> MGSSKPLKGFVICCTSIDLKQRTEISTKATKLGAAYRSDFTKDVTHLIAGDFDTPKYKFAAKSRPDIKIMSSEWIPVLYESWVQGEDLDDGLLVDKHLLPTLFKCRVCLTNIGQPERSRIENYVLKHGGTFCPDLTRDVTHLIAGTSSGRKYEYAL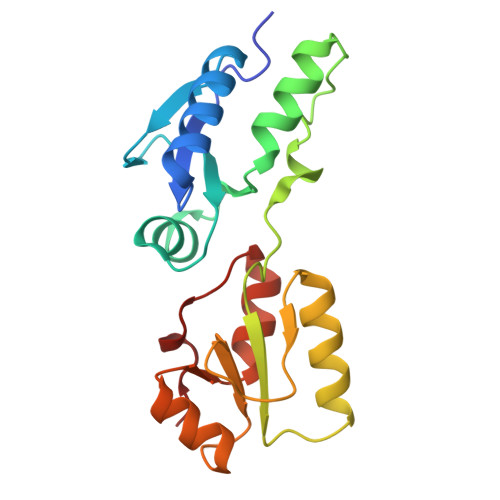KWKINVVCVEWLWQSIQRNAVLEPQYFQLD In addition, a much wider variety of ribozyme activities not found in nature have been discovered by in vitro evolution, including polymerase ribozymes (PR) that are capable of synthesizing a complementary strand on an RNA template. Recently, a variant utilizing trinucleotide triphosphates (triplets) as substrates [a triplet polymerase ribozyme (TPR)] was discovered. This TPR emerged as a heterodimer from in vitro evolution and displayed a remarkable ability to copy structured RNA templates including segments of its own sequence as well as circular RNA templates by rolling circle synthesis. Here, we report the cryogenic electron microscopy (cryo-EM) structure of an active PR, specifically the complete, heterodimeric TPR apoenzyme determined at its optimal functional magnesium ion concentration ([Mg2+] = 100 mM), augmented by a comprehensive fitness landscape of TPR function.

In this experiment, we identified two activity-enhancing mutations in t5 (ΔU38 and C110U) and combined them with three more t5 mutations (U117C, U132C, and U148A) identified in separate selection experiments (to be described elsewhere). This t5 (ΔU38, C110U, U117C, U132C, and U148A) variant was named 5TU and exhibited superior triplet polymerase activity. We obtained a 5.0-Å map of the TPR heterodimer apoenzyme with a local resolution varying from 5 to 9 Å (EMD-40984), indicative of high flexibility of some ribozyme domains. The model revealed the overall structural anatomy of the TPR to resemble an upturned left hand, with the thumb formed by the t1 subunit and fingers formed by the 5TU subunit at an approximate angle of 70°, and the palm formed by a bipartite interaction of the subunits through two distinct kissing loops (KL1, KL2). A striking feature of the TPR structure is that the two divergent subunits are held together by two distinct KL (KL1 and KL2) interactions (see model in cryo-EM map in SI Appendix). The structure of KL1 shows a 6-bp interaction between the loop of the 5TU:P1 hairpin and the t1:J1/2 internal loop, which results in a coaxial stack of 5TU:P1, the KL, and the t1:P2 stems. The structure of KL2 is a 2-bp loop-loop interaction between the identical apical loops of 5TU:P7 and t1:P3. The geometry created by these two KL interactions enforces a rigid, extended conformation of the single-stranded 5TU:J1/3 segment that is clearly visible in reconstructions from all our datasets. The 5TU core domain is found to have a similar overall conformation to cIL despite several mutations and the lack of the substrate helices. The core domain of t1 now forms an extended structure forming an L-shape (see model in cryo-EM map in SI Appendix) supported by positive epistasis values in our fitness landscape analysis. The t1:P1 helix appears to be supported at its base by two key tertiary interactions (the KL1 and A-anchor) that form a hinge allowing the large dynamic movement of t1:P1.

> GACCAAUCUGCCCUCAGAGCUCGAGAACAUCUUCGGAUGCAGAGGAGGCAGGCUUCGGUGGCGCGAUAGCGCCAACGUCCUCAACCUCCAAUGCAUCCCACCACAUGAUGAUGCCUGAAGAGCCUUGGUUUUUUG;> GGAUCUUCUCGAUCUAACAAAAAAGACAAAUCUGCCACAAAGCUUGAGAGCAUCUUCGGAUGCAGAGGCGGCAGCCUUCGGUGGCGCGAUAGCGCCAACGUUCUCAACUAUGACACGCAAAACGCGUGCUCCGUUGAAUGGAGUUUAUCAUG The biocatalytic reduction of the oxime moiety to the corresponding amine group has only recently been found to be a promiscuous activity of ene-reductases transforming α-oximo β-keto esters. By studying the crystal structures of enzyme oxime complexes, analyzing molecular dynamics simulations, and investigating biocatalytic cascades and possible intermediates, we obtained evidence that the reaction proceeds via an imine intermediate and not via the hydroxylamine intermediate. To gain more insight into the reaction pathway, we determined the crystal structures of the two enzymes OPR3 and XenA in complex with the oxime substrates 1a–c, either by co-crystallization or by soaking. All the crystal structures obtained had a high resolution (1.9–1.35 Å) and showed clear electron density features for the oximes.

To assess if the introduced amino acid exchanges affected the overall structure and the binding of the oxime, we also crystallized the tyrosine variants in complex with selected oxime substrates. The protomers in the crystal structures of the tyrosine variants are perfectly superimposable with the ones of the wild-type enzymes, confirming that the exchanges did not lead to major structural alterations. Interestingly, the binding mode of the oxime substrates also did not change in most of the structures. The propanoyl moiety of oxime 1b points into this cavity and is likely stabilized by hydrophobic interactions. Substrates with an acetyl moiety (such as oximes 1a and 1c) give the non-productive binding mode described above. It must be emphasized that such a residue (like Y27 in XenA) has never been proposed to be involved in a reaction mechanism of these enzymes. Previous experiments with XenA Y27F showed no involvement in the oxidative half-reaction. Looking at the results obtained for XenA, product formation was comparable for both tyrosine variants, the canonical Y183F and the non-canonical one (Y27F). The calculated high Kd for oxime 1b clearly indicates this enzyme’s low affinity for the substrate and might explain why this enzyme performed poorly in the biotransformation of the other oximes in our previous work. Both the Y183F and the Y27F variants of XenA showed a non-Michaelis–Menten behavior, with a linear increase of the rate over the concentration (bottom right).

>[2x]MSALFEPYTLKDVTLRNRIAIPPMCQFMAEDGLINDWHQVHYASMARGGAGLLVVEATAVAPEGRITPGCAGIWSDAHAQAFVPVVQAIKAAGSVPGIQIAHAGRKASANRPWEGDDHIGADDARGWETIAPSAIAFGAHLPNVPRAMTLDDIARVKQDFVDAARRARDAGFEWIELHFAHGYLGQSFFSEHSNKRTDAYGGSFDNRSRFLLETLAAVREVWPENLPLTARFGVLEYDGRDEQTLEESIELARRFKAGGLDLLSVSVGFTIPETNIPWGPAFMGPIAERVRREAKLPVTSAWGFGTPQLAEAALQANQLDLVSVGRAHLADPHWAYFAAKELGVEKASWTLPAPYAHWLERYRLEHHHHHH>[2x]GASSSSESLSIIDVASDQNLFQTFIKEWRCKKRFSISLACEKIRSLTSSKTGFPIKGCDDTLVVGLAVCWGGRDAYYFSLQKESLDPSLTLKDRMWYLQSCLRKESDKECSVVIYDFIQSYKILLLSCGISLEQSYEDPKVACWLLDPDSQEPTLHSIVTSFLPHEL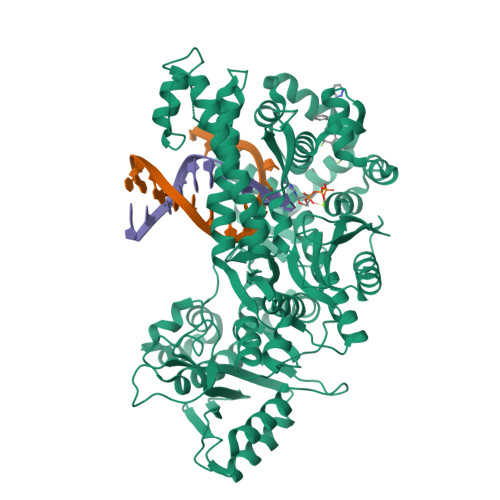PLLEGMETSQGIQSLGLNAGSEHSGRYRASVESILIFNSMNQLNSLLQKENLQDVFRKVEMPSQYCLALLELNGIGFSTAECESQKHIMQAKLDAIETQAYQLAGHSFSFTSSDDIAEVLFLELKLPPNRELGRQFSTSKDVLNKLKALHPLPGLILEWRRITNAITKVVFPLQREKCLNPFLGMERIYPVSQSHTATGRITFTEPNIQNVPRDFEIKMPTLADRGMPFSISMRHAFVPFPGGSILAADYSQLELRILAHLSHDRRLIQVLNTGADVFRSIAAEWKMIEPESVGDDLRQQAKQICYGIIYGMGAKSLGEQMGIKENDAACYIDSFKSRYTGINQFMTETVKNCKRDGFVQTILGRRRYLPGIKDNNPYRKAHAERQAINTIVQGSAADIVKIATVNIQKQLETFHSTFKSHGHREGMLQSDQTGGMFCPIRGGFFILQLHDELLYEVAEEDVVQVAQIVKNEMESAVKLSVKLKVKVKIGASWGELKDFDV> DITFRNIRFRYKPDSPVILDNINLSIKQGEVIGIVGRSGSGKSTLTKLIQRFYIPENGQVLIDGHDLALADPNWLRRQVGVVLQDNVLLNRSIIDNISLANPGMSVEKVIYAAKLAGAHDFISELREGYNTIVGEQGAGLSGGQRQRIAIARALVNNPKILIFDEAT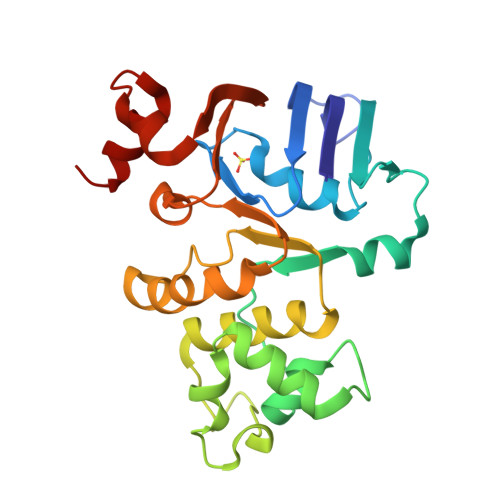SALDYESEHVIMRNMHKICKGRTVIIIAHRLSTVKNADRIIVMEKGKIVEQGKHKELLSEPESLYSYLYQLQSD N-[(benzyloxy)carbonyl]glycyl-N-[(2S,3R)-4-chloro-3-hydroxy-1-phenylbutan-2-yl]glycinamide 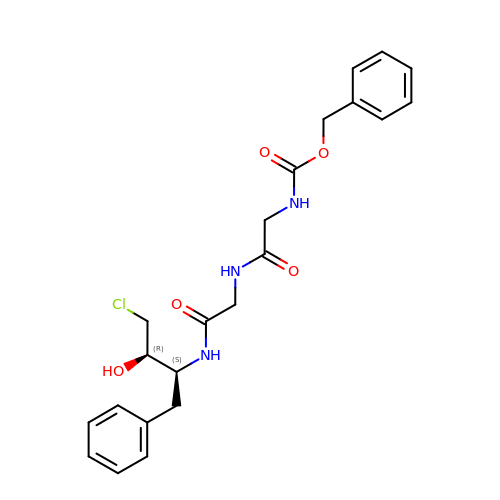| C22 H26 Cl N3 O5 | WLEADEPGUSFGIL-OALUTQOASA-N6-[1-(3,5,5,8,8-PENTAMETHYL-5,6,7,8-TETRAHYDRONAPHTHALEN-2-YL)CYCLOPROPYL]PYRIDINE-3-CARBOXYLIC ACID | C24 H29 N O2 | 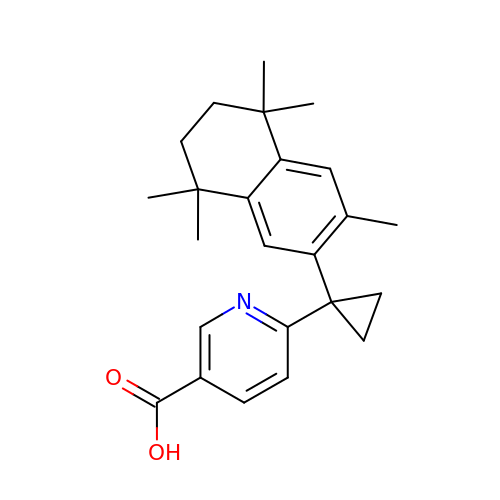SLXTWXQUEZSSTJ-UHFFFAOYSA-N>MIHHHHHHEHRHLKPFPPEFLWGAASAAYQVEGAWNEDGKGLSVWDVFAKQPGRTFKGTNGDVAVDHYHRYQEDVALMAEMGLKAYRFSVSWSRVFPDGNGAVNEKGLDFYDRLIEELRNHGIEPIVTLYHWDVPQALMDAYGAWESRRIIDDFDRYAVTLFQRFGDRVKYWVTLNEQNIFISFGYRLGLHPPGVKDMKRMYEANHIANLANAKVIQSFRHYVPDGKIGPSFAYSPMYPYDSRPENVLAFENAEEFQNHWWMDVYAWGMYPQAAWNYLESQGLEPTVAPGDWELLQAAKPDFMGVNYYQTTTVEHNPPDGVGEGVMNTTGKKG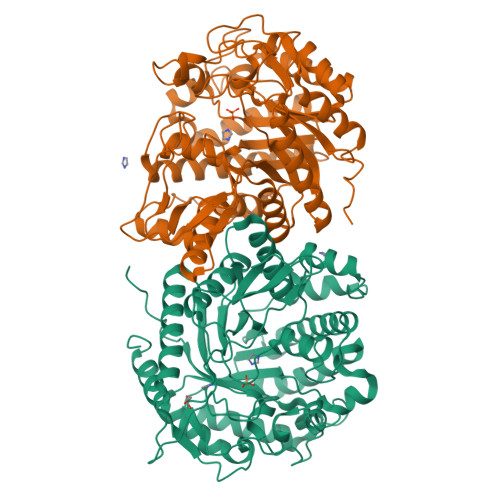TSTSSGIPGLFKTVRNPHVDTTNWDWAIDPVGLRIGLRRIANRYQLPILITENGLGEFDTLEPGDIVNDDYRIDYLRRHVQEIQRAITDGVDVLGYCAWSFTDLLSWLNGYQKRYGFVYVNRDDESEKDLRRIKKKSFYWYQRVIETNGAEL[4x]> EAASSSDADGKEVGSSGEGNRATGGKWRRPSLAQQRARRAQLPPAFDVVHWNDEDISRGHLLRVLHRDTFVVLDYHRQARMLTEEGNKAERVVSVMLPAVYTARFLAVLEGRSEKVEVHSRYTNATFTPNPAAPYTFTLK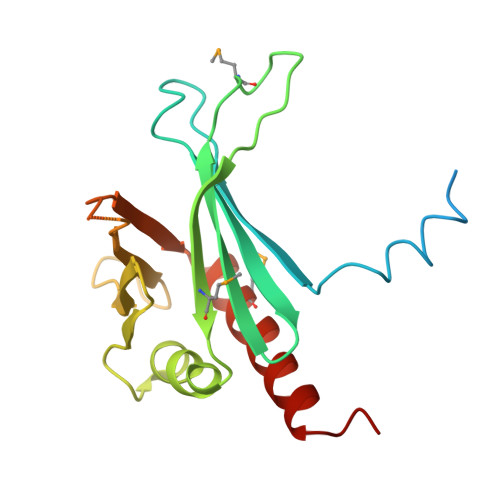CTSTRPAQQKQQVAGEEGDETFEWTVEFDVAESLMLQRFLTQALHYNTGFARTSV LDH and MDH are homologous, 2-ketoacid oxidoreductases that share both a protein fold (Rossmann et al., 1975) and a common catalytic mechanism (Birktoft and Banaszak, 1983; Clarke et al., 1986; Hart et al., 1987a, 1987b; Clarke et al., 1988; Waldman et al., 1988). Both enzymes are found in central metabolism: MDH catalyzes the interconversion of oxaloacetate and malate in the citric acid cycle, and LDH converts pyruvate to lactate in the final step of anaerobic glycolysis. A key event in the early evolution of the Apicomplexa was the acquisition of a malate dehydrogenase (MDH) via lateral gene transfer from α-proteobacteria. Following a gene duplication event roughly 700–900 Mya, one copy of this MDH evolved a novel substrate specificity to become a highly specific lactate dehydrogenase (LDH) that is now essential to the life cycle of many modern apicomplexans.

In order to understand the structural changes during evolution that shifted the enzymatic substrate specificity of the apicomplexan dehydrogenases, we determined the high-resolution crystal structures of three ancestral proteins bracketing the key duplication event: AncMDH2, AncLDH*, and AncMDH2-INS. Each protein was crystallized with multiple substrates or ligands (lactate, malate, and oxamate inhibitor) and with NADH (resolution ranging from 1.35 Å to 2.05 Å). In the following, therefore, the descriptions of the models are primarily based on enzymes crystallized with oxamate inhibitor or lactate, which are highly similar. AncMDH2* is a strict MDH, and AncLDH* is a strict LDH. The ancestral AncLDH* and modern apicomplexan LDH structures are likewise highly similar (Winter et al., 2003; Cameron et al., 2004; Kavanagh et al., 2004) (RMSD ∼0.8 Å for the loop-closed states), while sharing only 63–71% sequence identity. The first shell active site residues are identical in the AncLDH* and modern Toxoplasma LDHs, comprising the same residues as the apicomplexan MDH active site with the sole exception of position 102, which is replaced by Trp107f in the LDHs. The conformations of the ancestral and modern active sites are nearly indistinguishable, with only small differences in the specificity loop conformation. In both the ancestral and modern LDH structures, Trp107f and Arg109 are the only residues from the specificity loop that interact with the substrate. As in the modern LDH structures, ancestral Lys102 does not interact with the substrate but points away from the active site into solution. In contrast, Trp107f is buried within the active site, with the edge of the indole ring interacting with the pyruvate C3 methyl, which is the very chemical moiety that distinguishes pyruvate from oxaloacetate.

>[2x]MTGTMTKRKKISLIGSGMIGGTMAYLCAQKELGDVVLFDVVKNMPQGKALDLSHSSSIADTNVKVTGTNSYEDIKGSDVVIITAGLTKAPGKSDKEWSRDDLLPFNAKIMREVGENIKKYCPNAFVIVITNPLDVMVKVLHEHSGLPKNKVCGMAGVLDSSRFRHFIAEKLNVSPRDVQAMVIGAHGDKMVPLTRYVTVNGIPLQEFIKKGRITQEEIDEIVERTKNAGGEIVNLLGQGSAYFAPAASAIEMAEAYLKDKKRVLVCSCYLEGQYGHKDMFVGVPAVIGGNGVEKVIELELTPEEKELFDKSVEEVRKLQKAIKALGLEHHHHHH> DLENLYF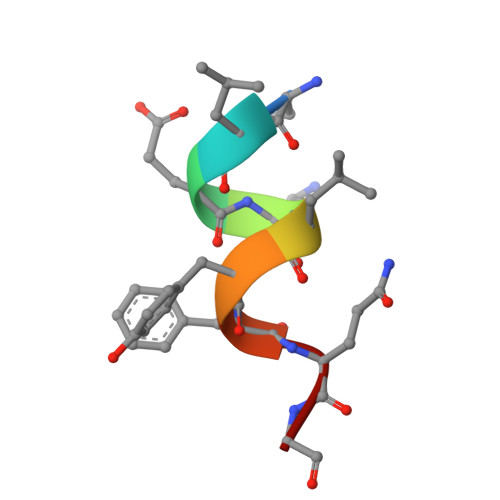QG> MSQQAPDPAIRAALQSQPSGLASDDWEAAMQRIMALTTRNPESFRQQPQANRLSAILEAVVPSRTNPTHEKVLAIVNALAENKAIRPDEAGLVYNALLERVGRYNSTNVQSNLDRLVTDVREAVAQRERFKNEGLGSLVALNAFLATQPANVPRGQDDYTNFISALRLMVTEVPQSEVYQSGPDYFFQTSRQGLQTVNLSQAFKNLRGLWGVQAPVGDRSTVSSLLTPNSRLLLLLIAPFTD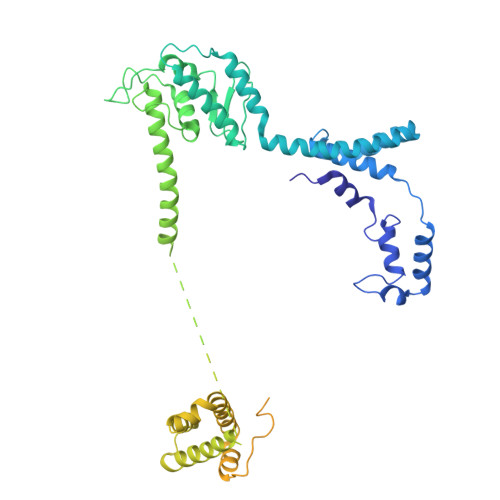SGSVNRNSYLGHLLTLYREAIGQAQVDEQTFQEITSVSRALGQNDTDSLRATLNFLLTNRQQKIPAQYALSAEEERILRYVQQSVGLFLMQEGATPSAALDMTARNMEPSMYAANRPFINKLMDYLHRAAAMNTDYFTNAILNPHWLPPPGFYTGEYDMPDPNDGFLWDDVDSAVFSPTFQKRQEAPPSEGAVGRSPFPSLGSLHSLPGSVNSGRVSRPRLLGEDEYLNDSLLQPPRAKNAMANNGIESLVDKLNRWKTYAQDHRDAPAPRRQRHDRQRGLVWDDEDSADDSSVLDLGGSGGVNPFAHLQPKLGRRMF> MEWSQIFHDITTKHDFKAMHDFLEKEYSTAIVYPDRENIYQAFDLTPFENIKVVILGQ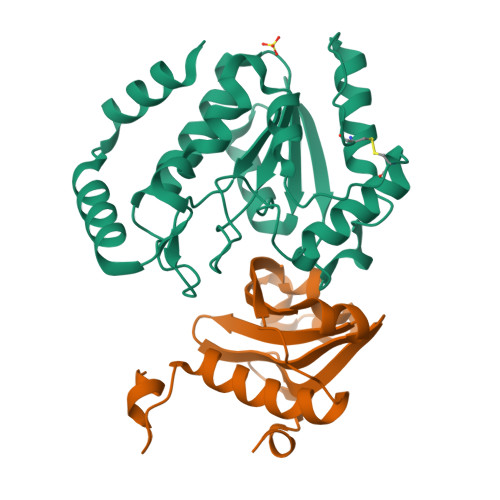DPYHGPNQAHGLAFSVQPNAKFPPSLRNMYKELADDIGCVRQTPHLQDWAREGVLLLNTVLTVRQGEANSHRDIGWETFTDEIIKAVSDYKEHVVFILWGKPAQQKIKLIDTSKHCIIKSVHPSPLSAYRGFFGSKPYSKANTYLESVGKSPINWCESEALEHHHHHH;> HHHHHHSSGLVPRGSHMKTTTQELKQYMTRLFQLSNNETWECETLEEAAENILPKRFINDSPLAHLILETYTYYNNELHELSIYPFLMYSNNQLISIGYLDHFDMDFLYLTDTKNTIIDERHLLKEGGNNHE> MKITSSNFATIA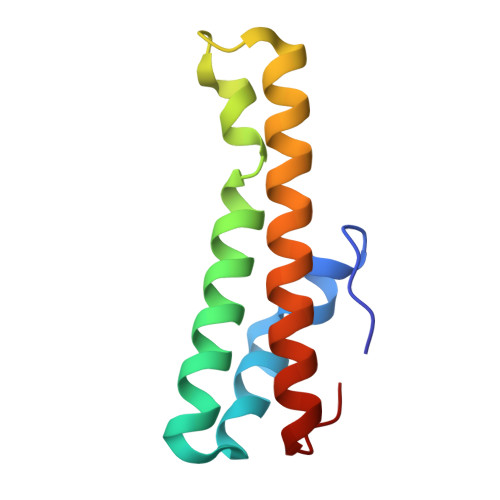TSENFAKLSVLPKNHREPIKGLFKSAVEQFSSARDFFKNENYSKELAEKFNKEAVNEAVEKLQKAIDLAEKQGIQF>MKASKLSCLGLIGVIPACIHAQEHRADDTLRPNIIYIFPDQMRNSAMGFWNDPAFASHLQGKADPVETPNLNRFARESVVFSSAMSNCPLSSPHRASLLTGMYPHRSGVPLNVNSRRPFSTLRNDATTVSDVFSRNGYDCAYIGKYHL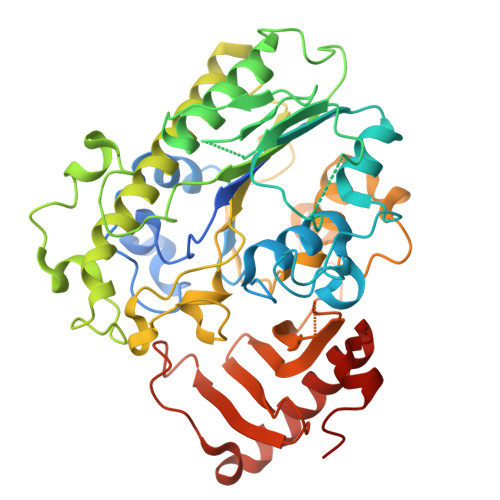DTPTPNDPENPGNYVENRDLVWDAYTPPERRHGFNFWYSYGTFDVHKHPHYWDTDGKRHDINQWSPSHETDMAISYLKNEFGRRDVSKPFFLMISMNPPHHPYNSFNDCMEEDYTHYKDRTLSELLVRHNADTTMEKSSSAAYYFAQITGVDREFGRLLEALDELGLSKNTMVVFSSDHGETMCSHGLQDAKNSPYIESMNVPFLIRYPQRLKPKVVDYLLSSPDIMPTLLGLSNLGQHIPHEVQGTDFSKALFSNQPDKPLPDAALYIRNMDGRQDQDGKVRTYVPVARGIKTHRYTLSLTVDKENKQLKEILLFDDLDDPYQMNNIDWNTRPQLKRQLLIQLGQLLKKYDDPWYKDGILKDLIMYE[3x]>GSHMGQSLRTLQGHQSAVTSLQFNDNIVVSGSDDSTVKVWDIKTGQSLRTLQGHQSA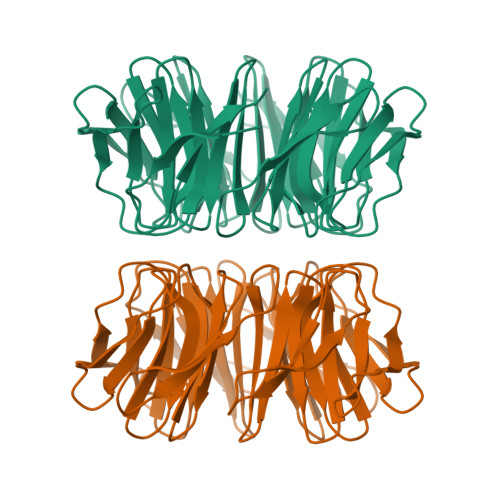VTSLQFNDNIVVSGSDDSTVKVWDIKTGQSLRTLQGHQSAVTSLQFNDNIVVSGSDDSTVKVWDIKTGQSLRTLQGHQSAVTSLQFNDNIVVSGSDDSTVKVWDIKTGQSLRTLQGHQSAVTSLQFNDNIVVSGSDDSTVKVWDIKTGQSLRTLQGHQSAVTSLQFNDNIVVSGSDDSTVKVWDIKTGQSLRTLQGHQSAVTSLQFNDNIVVSGSDDSTVKVWDIKTGQSLRTLQGHQSAVTSLQFNDNIVVSGSDDSTVKVWDIKGS[2x]4-{[(1S,2S)-2-(carboxymethyl)cyclopentyl]methyl}benzoic 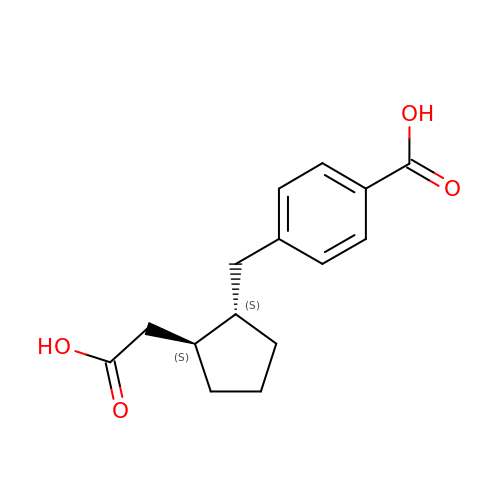acid | C15 H18 O4 | MXTHRYIVPLVGFC-STQMWFEESA-N>MVTYTTLLDKPISESAPRKAPEPLLREALGAALRSFRADKGVTLRELAEASRVSPGYLSELERGRKEVSSELLASVCHALGASVADVLIEAAGSMALQAAQEDLARVLEWSHPQ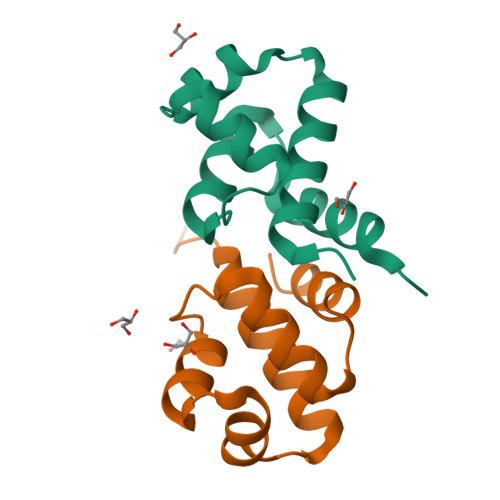FEK[2x]>[2x]MAMHPRKDWYELTRATNWTPSYVTEEQ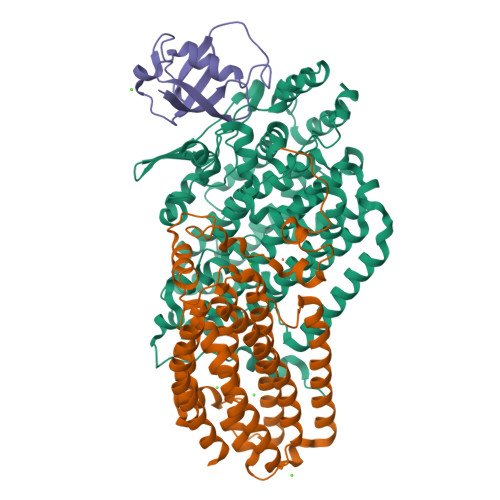LFPERMSGHMGIPLEKWESYDEPYKTSYPEYVSIQREKDAGAYSVKAALERAKIYENSDPGWISTLKSHYGAIAVGEYAAVTGEGRMARFSKAPGNRNMATFGMMDELRHGQLQLFFPHEYCKKDRQFDWAWRAYHSNEWAAIAAKHFFDDIITGRDAISVAIMLTFSFETGFTNMQFLGLAADAAEAGDYTFANLISSIQTDESRHAQQGGPALQLLIENGKREEAQKKVDMAIWRAWRLFAVLTGPVMDYYTPLEDRSQSFKEFMYEWIIGQFERSLIDLGLDKPWYWDLFLKDIDELHHSYHMGVWYWRTTAWWNPAAGVTPEERDWLEEKYPGWNKRWGRCWDVITENVLNDRMDLVSPETLPSVCNMSQIPLVGVPGDDWNIEVFSLEHNGRLYHFGSEVDRWVFQQDPVQYQNHMNIVDRFLAGQIQPMTLEGALKYMGFQSIEEMGKDAHDFAWADKCKPAMKKSA;>[2x]MSFESKKPMRTWSHLAEMRKKPSEYDIVSRKLHYSTNNPDSPWELSPDSPMNLWYKQYRNASPLKHDNWDAFTDPDQLVYRTYNLMQDGQESYVQSLFDQFNEREHDQMVREGWEHTMARCYSPLRYLFHCLQMSSAYVQQMAPASTISNCCILQTADSLRWLTHTAYRTHELSLTYPDAGLGEHERELWEKEPGWQGLRELMEKQLTAFDWGEAFVSLNLVVKPMIVESIFKPLQQQAWENNDTLLPLLIDSQLKDAERHSRWSKALVKHALENPDNHAVIEGWIEKWRPLADRAAEAYLSMLSSDILPAQYLERSTSLRASILTV;>[2x]MSAFPVHAAFEKDFLVQLVVVDLNDSMDQVAEKVAYHCVNRRVAPREGVMRVRKHRSTELFPRDMTIAESGLNPTEVIDVVFEE>LGINCRGSSQCGLSGGNLMV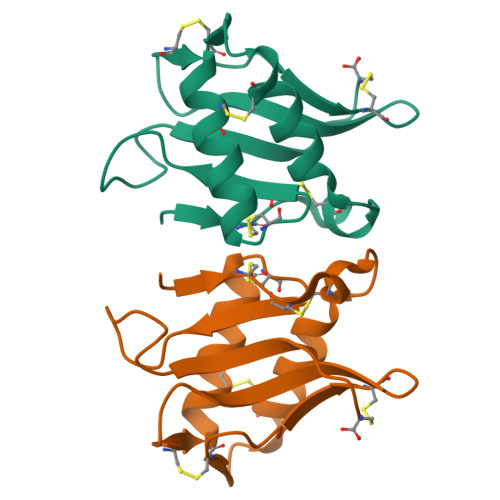RIRDQACGNQGQTWCPGERRAKVCGTGNSISAYVQSTNNCISGTEACRHLTNLVNHGCRVCGSDPLYAGNDVSRGQLTVNYVNSC[2x]>AYMFSDRSTSLSIEEERFLDAAEYGNIPVVRKMLEECHSLNVNCVDYMGQNALQLAVANEHLEITELLLKKENLSRVGDALLLAISKGYVRIVEAILSHPAFAEGKRLATSPSQSELQQDDFYAYDEDGTRFSHDVTPIILAAHCQEYEIVHTLLRKGARIERPHDYFCKCNDCNQKQKHDSFSHSRSRINAYKGLASPAYLSLSSEDPVMTALELSNELAVLANIEKEFKNDYKKLSMQCKDFVVGLLDLCRNTEEVEAILNGDVETLQSGDHGRPNLSRLKLAIKYEVKKFVAHPNCQQQLLSIWYENLSGLRQQTMAVKFLVVLAVAIGLPFLALIYWFAPCSKMGKIMRGPFMKFVAHAASFTIFLGLLVMNAADRFEGTKLLPNETSTDNAKQLFRMKTSCFSWMEMLIISWVIGMIWAECKEIWTQGPKEYLFELWNMLDFGMLAIFAASFIARFMAFWHASKAQSIIDANDTLKDLTKVTLGDNVKYYNLARIKWDPSDPQIISEGLYAIAVVLSFSRIAYILPANESFGPLQISLGRTVKDIFKFMVIFIMVFVAFMIGMFNLYSY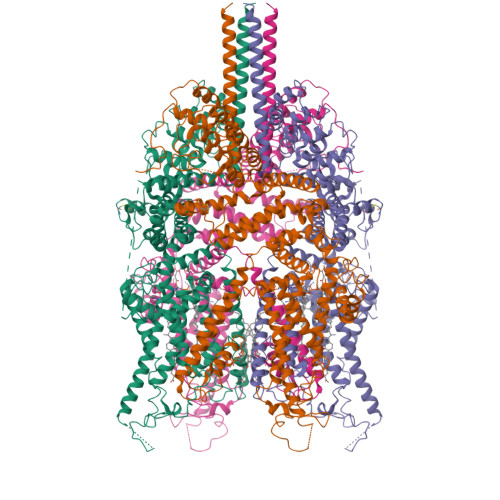YIGAKQNEAFTTVEESFKTLFWAIFGLSEVKSVVINYNHKFIENIGYVLYGVYNVTMVIVLLNMLIAMINSSFQEIEDDADVEWKFARAKLWFSYFEEGRTLPVPFNLVPSPKSLFYLLLKLKKWISELFQGHKKGFQEDAEMNKINEEKKLGILGSHEDLSKLSLDKKQVGHNKQPSIRSSEDFHLNSFNNPPRQYQKIMKRLIKRYVLQAQIDKESDEVNEGELKEIKQDISSLRYELLEEKSQNTEDLAELIRELGEKLSMEPNQEETNR[4x]> MGAVFDRRAFLLTLGSLVFLPAGAARAAGLDAAAAATRLAAIETSLDGRLGLFALNTADGRTLAHRSDERFAMCSTFKLVLAGAILAQSAQTPGLLERRVAYGPEALVSYSPITQKHAAGGM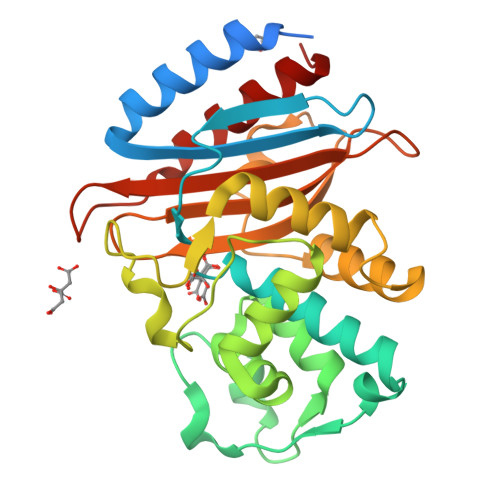TVAALCAAAVRHSDNTAANLLLDQLDGPAALTTFARTIGDNHFRLDRREPELNTAIPGDPRDTTTPAAMGRSLQRLALGRALPAEGRALLCAWLRGCVTGAARIRAGVPAGWVVGDKTGTGAYGVANDVAVLWPAAGAPPVLLAIYTARRQKDAAPRNDVIVAAAKVVAEWLGAAA methyl 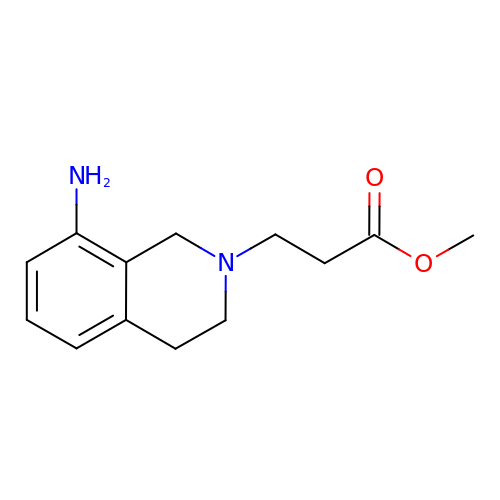3-(8-amino-3,4-dihydroisoquinolin-2(1H)-yl)propanoate | C13 H18 N2 O2 | HYEBSCFAHVBELO-UHFFFAOYSA-N> MRGGALLCGQVQDEIEQLSRESSHFSLSTGILPSLGARSNRRVKLRRFVVSPYDHKYRIWEAFLVVLVVYTAWVSPFEFGFLRKPRPPLSITDNIVNAFFAIDIIMTFFVGYLDKSTYLIVDDRKQIAFKYLRSWFLLDLVSTIPSEAAMRISSQSYGLFNMLRLWRLRRVGALFARLEKDRNFNYFWVRCAKLVCVTLFAVHCAACFYYLIAARNSNPAKTWIGANVANFLEESLWMRYVTSMYWSITTLTTVGYGDLHPVNTKEMIFDIFYMLFNLGLTAYLIGNMTNLVVHGTSRTRNFRDTIQAASNFAHRNHLPPRLQDQMLAHLCLKYRTDSEGLQQQETLDALPKAIRSSISHFLFYSLMDKVYLFRGVSNDLLFQLVSEMKAEYFPPKEDVILQNEAPTDFYILVNGTADLVDVDTGTESIVREVKAGDIIGEIGVLCYRPQLFTVRTKRLCQLLRMNRTTFLNIIQANVGDGTIIMNNLLQHLKEMNDPVMTNVLLEIENMLARGKMDLPLNLCFAAIREDDL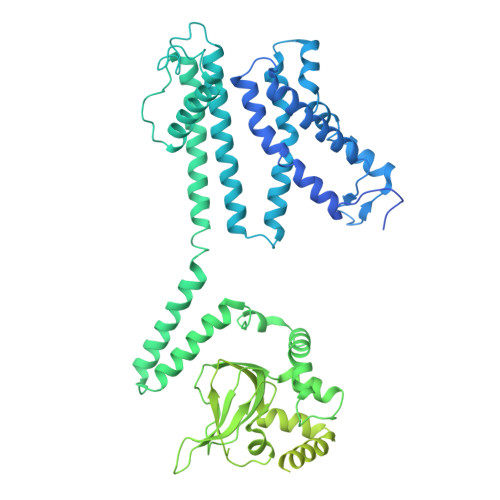LLHQLLKRGLDPNESDNNGRTPLHIAASKGTLNCVLLLLEYHADPNCRDAEGSVPLWEAMVEGHEKVVKVLLEHGSTIDAGDVGHFACTAAEQGNLKLLKEIVLHGGDVTRPRATGTSALHTAVCEENIEMVKYLLEQGADVNKQDMHGWTPRDLAEQQGHEDIKALFREKLHERRVHIETSSSVPILKTGIRFLGRFTSEPNIRPASREVSFRIRETRARRKTNNFDNSLFGILANQSVPKNGLATVDEGRTGNPVRVTISCAEKDDIAGKLVLLPGSFKELLELGSNKFGIVATKVMNKDNNAEIDDVDVIRDGDHLIFATDSLEGSDEVDAGSAAASGGSGSDYKDDDDK> MVFEFLFYNQQHKTRNGYFINHDNLMLASLEERKKLIFYFIANQVPEKLDPVDRVKFNEELSDNLSTKARLIGSLTG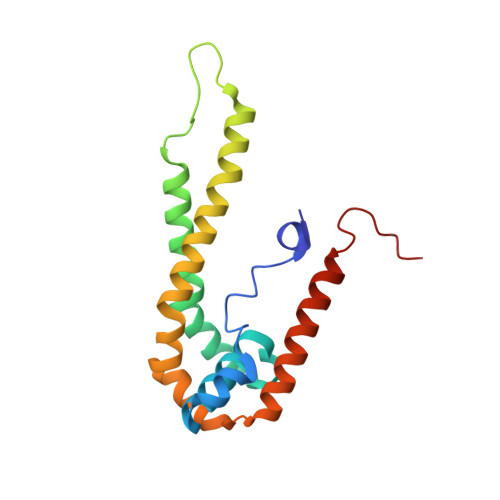LIGLVGFPYISTRIYSRPVLNIGLSLLICPFLYYVGNQLTYSVWEPKFIANNNTVCELSKKYNFTVFDFAQAKKEAHLKALRTELVSDNLLYSPGI> NICEITEVDSTLVERLGQRLLPWMDRLSQEQLNPSIYVGLRLSSLQAGAKEAHYLHSLKLSYQQSLLRPASNKDDNDSEAKPSMGQLALYLLALRANCEFIGGRKGDRLVSQLKRFLEDEKRAIGHNHQGHPRTSYYQYSLGILALCVHQKRVHDSVVGKLLYAVEHKPHLLQDHVSVDTMAMAGMAFSCLELSNLNPKQRNRINLALKRVQEKILKAQT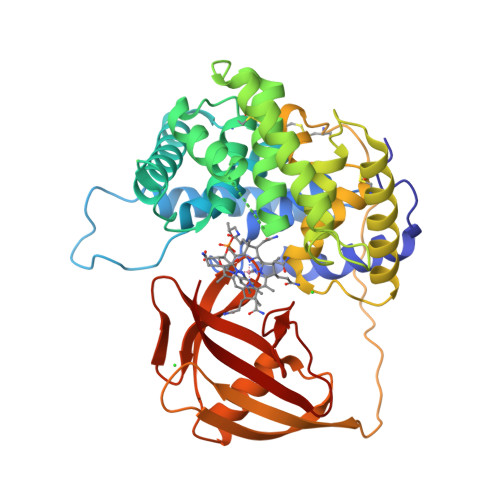PEGYFGNVYSTPLALQLLMGSLRPSVELGTACLKAKAALQASLQHKTFQNPLMISQLLPVLNQKSYVDLISPDCQAPRALLEPALETPPQAKVPKFIDVLLKVSGISPSYRHSVSVPAGSSLEDILKNAQEHGRFRFRTQASLSGPFLTSVLGRKAGEREFWQVLRDPDTPLQQGIADYRPKDGETIELRLVGW> METKLTYGNRVTLPEFAKYIVAPAFHEIEGRAIPVTGVDDDASGTQATKLPFVLVG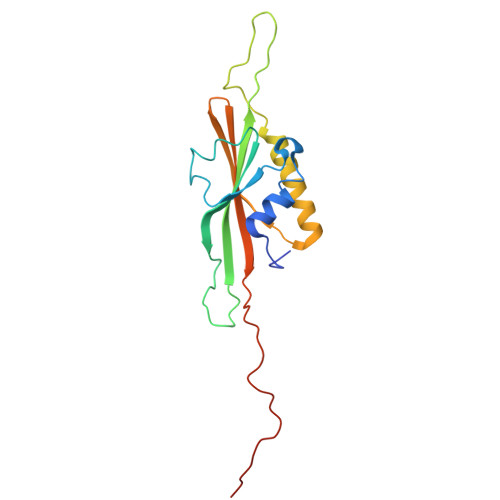LRQGDTSGPATIAGNSTINLRDDFIVEFNMKKERYRDRKGGETPFFSYYDYESIRDRLFNSMIEFSGEHGITFEFVSLDISTEGDVVYIEFRFRQNYEWCETVREADTTIEAGRFSINLQGC>[4x]GDTKEQRILRYVQQNAKPGDPQSVLEAIDTYCTQKEWAMNVGDAKGQIMDAVIREYSPSLVLELGAYCGYSAVRMARLLQPGARLLTMEINPDCAAITQQ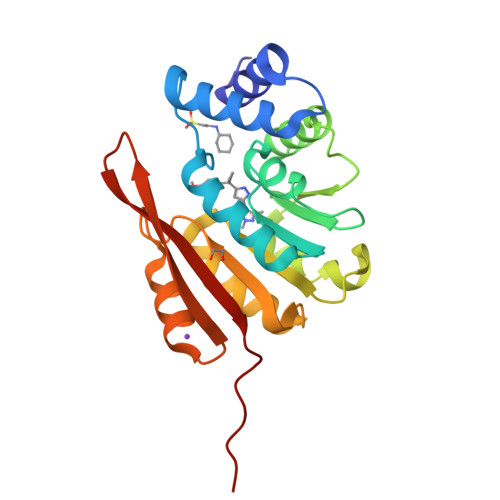MLNFAGLQDKVTILNGASQDLIPQLKKKYDVDTLDMVFLDHWKDRYLPDTLLLEKCGLLRKGTVLLADNVIVPGTPDFLAYVRGSSSFECTHYSSYLEYMKVVDGLEKAIYQGPSSPDKS>MLSRKGIIPEEYVLTRLAEDPTEPRYRTRERRARFVSKKGNCNVAHKNIRERGRFLQDVFTTLVDLKWPHTLLIFTMSFLCSWLLFAMVWWLIAFAHGDLAPGEGTNVPCVTSIHSFSSAFLFSIEVQVTIGFGGRMVTEECPLAILILIVQNIVGLMINAIMLGCIFMKTAQAHRRAETLIFSKHAVITLRHGRLCFMLRVGDLRKSMIISATIHMQVVRKTTSPEGEVVPLHQVDIPMENGVGGNSIFLVAPLIIYHVIDSNSPLYDLAPSDLHHHQDLEIIVILEGVVETTGITTQARTSYLADEILWGQRFVPIVAEEDGRYSVDYSKFGNTVKVPTPLCTARQLDEDRSLLDALTLASSRGPLRKRSVAVAKAKPKFSISPDSLS[4x];>MPLAFCGTENHSAAYRVDQGVLNNGCFVDALNVVPHVFLLFITFPILFIGWGSQSSKVHIHHSTWLHFPGHNLRWILTFILLFVLVCEIAEGILSDGVTESRHLHLYMPAGMAFMAAITSVVYYHNIETSNFPKLLIALLIYWTLAFITKTIKFVKFYDHAIGFSQLRFCLTGLLVILYGMLLLVEVNVIRVRRYIFFKTPREVKPPEDLQDLGVRFLQPFVNLLSKGTYWWMNAFIKTAHKKPIDLRAIGKLPIAMRALTNYQRLCVAFDAQARKDTQSPQGARAIWRALCHAFGRRLILSSTFRILADLLGFAGPLCIFGIVDHLGKENHVFQPKTQFLGVYFVSSQEFLGNAYVLAVLLFLALLLQRTFLQASYYVAIETGINLRGAIQTKIYNKIMHLSTSNLSMGEMTAGQICNLVAIDTNQLMWFFFLCPNLWAMPVQIIVGVILLYYILGVSALIGAAVIILLAPVQYFVATKLSQAQRSTLEHSNERLKQTNEMLRGMKLLKLYAWESIFCSRVEVTRRKEMTSLRAFAVYTSISIFMNTAIPIAAVLITFVGHVSFFKESDLSPSVAFASLSLFHILVTPLFLLSSVVRSTVKALVSVKKLSEFLSSAEIREEQCAPREPAPQGQAGKYQAVPLKVVNRKRPAREEVRDLLGPLQRLAPSMDGDADNFCVQIIGGFFTWTPDGIPTLSNITIRIPRGQLTMIVGQVGCGKSSLLLATLGEMQKVSGAVFWNSNLPDSEGEDPSSPERETAAGSDIRSRGPVAYASQKPWLLNATVEENITFESPFNKQRYKMVIEACSLQPDIDILPHGDQTQIGERGINLSGGQRQRISVARALYQQTNVVFLDDPFSALDVHLSDHLMQAGILELLRDDKRTVVLVTHKLQYLPHADWIIAMKDGTIQREGTLKDFQRSECQLFEHWKTLMNRQDQELEKETVMERKASEPSQGLPRAMSSRDGLLLDEEEEEEEAAESEEDDNLSSVLHQRAKIPWRACTKYLSSAGILLLSLLVFSQLLKHMVLVAIDYWLAKWTDSALVLSPAARNCSLSQECDLDQSVYAMVFTLLCSLGIVLCLVTSVTVEWTGLKVAKRLHRSLLNRIILAPMRFFETTPLGSILNRFSSDCNTIDQHIPSTLECLSRSTLLCVSALTVISYVTPVFLVALLPLAVVCYFIQKYFRVASRDLQQLDDTTQLPLLSHFAETVEGLTTIRAFRYEARFQQKLLEYTDSNNIASLFLTAANRWLEVRMEYIGACVVLIAAATSISNSLHRELSAGLVGLGLTYALMVSNYLNWMVRNLADMEIQLGAVKRIHALLKTEAESYEGLLAPSLIPKNWPDQGKIQIQNLSVRYDSSLKPVLKHVNALISPGQKIGICGRTGSGKSSFSLAFFRMVDMFEGRIIIDGIDIAKLPLHTLRSRLSIILQDPVLFSGTIRFNLDPEKKCSDSTLWEALEIAQLKLVVKALPGGLDAIITEGGENFSQGQRQLFCLARAFVRKTSIFIMDEATASIDMATENILQKVVMTAFADRTVVTIAHRVHTILSADLVMVLKRGAILEFDKPETLLSQKDSVFASFVRADK[4x]

ATP-sensitive potassium (KATP) channels, composed of four pore-lining Kir6.2 subunits and four regulatory sulfonylurea receptor 1 (SUR1) subunits, control insulin secretion in pancreatic β-cells. KATP channel opening is stimulated by PIP2 and inhibited by ATP. Mutations that increase channel opening by PIP2 reduce ATP inhibition and cause neonatal diabetes. In addition to adenine nucleotides-dependent regulation, membrane phosphoinositides participate in the gating activation of KATP channels, as they do all other eukaryotic Kir channels.

Here, we present the cryoEM structure of the KATP channel harboring the neonatal diabetes Q52R mutation (hereinafter referred to as the SUR1/Kir6.2Q52R channel) in an open conformation bound to amphipathic molecules consistent with natural C18:0/C20:4 long-chain PI(4,5)P2. At each Kir6.2-SUR1 interface, one PIP2 molecule is bound within the site that is conserved among Kir channels (referred to as the canonical site), and a second PIP2 molecule is at an adjacent site, stacked within the regulatory interface between Kir6.2 and SUR1-TMD0 (referred to as the non-canonical site). First, C18:0/C20:4 PI(4,5)P2 is the dominant species in the brain PIP2 present in our sample (~75%), and both amphipathic molecule densities have map features for the phospho-head groups as well as long acyl chains consistent with C18:0/C20:4 PI(4,5)P2 (monomer ID PT5). In addition to lipid densities at the SUR1-Kir6.2 interface, three other well-resolved lipid map features at the inner leaflet of the membrane bilayer were bound between SUR1-TMD0 and SUR1-TMD1. These were best modeled by the common phospholipids phosphatidylethanolamine and phosphatidylserine. The structure of the PIP2-bound SUR1/Kir6.2Q52R channel has an open Kir6.2 inner helix gate. In the PIP2-bound open SUR1/Kir6.2Q52R structure, the two NBDs of SUR1 are not well resolved; in particular, NBD2 is highly dynamic with a local resolution > 5 Å. However, the two NBDs are clearly separated, as predicted since no MgATP or MgADP was added to the sample. The ABC modules of the four SUR1 subunits in the PIP2-bound open SUR1/Kir6.2Q52R map from a C4 non-uniform refinement adopt a propeller-like conformation. Further 3D classification of the symmetry-expanded particle set revealed three distinct rotational positions of the SUR1-ABC module relative to the Kir6.2/SUR1-TMD0 tetrameric core.>[10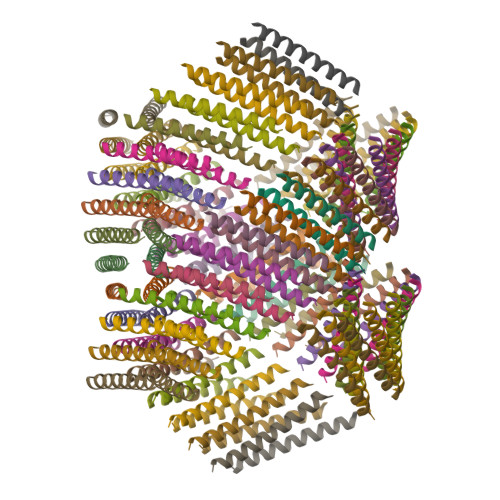4x]QAEILKADAEILKAYAKILEAHAEILKAQ4,4'-Diaponeurosporene | C30 H42 | 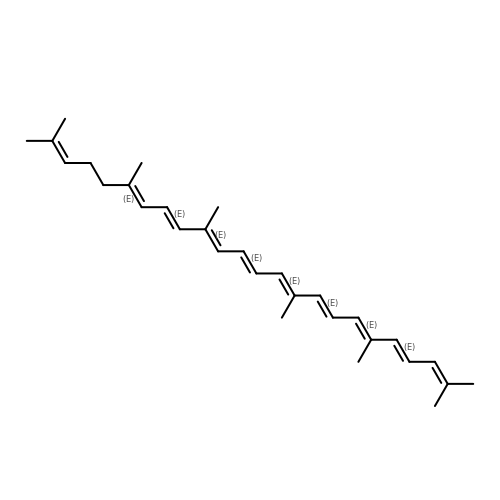FPSYVUBUILNSRF-MQMKOTMBSA-N>[3x]MRRGSGNPERPSLSRDGLRVPPPCPGKRGPGH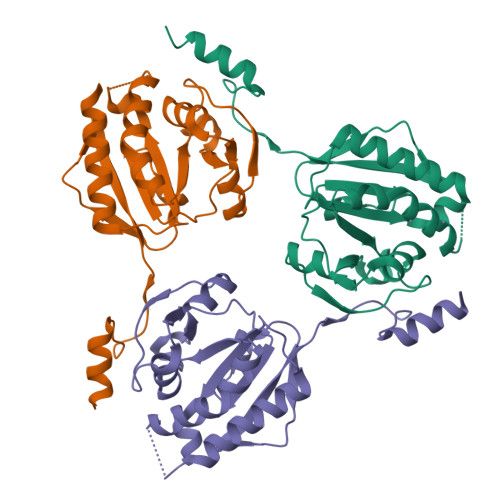FSGYHGGMEGIRRAAQRAAEEFLQAFPMAPGSLFVLGGSTSEVLGERVGTRPSLEAAHAVLEGLLPPLLERGVHVAVQACEHLNRALVVERETARAFGKEEVAVFPHPKAGGAKATAAFLRFRDPVMVESLKAQAHGGMDIGGVLIGMHLRPVAVPLRLSVRKIGEAVLLAAKTRPKLVGGARAVYTREEMLKKLEEFLPKPP> MDVVSLDKPFMYFEEIDNELDYEPESANEVAKKLPYQGQLKLLLGELFFLSKLQRHGILDGATVVYIGSAPGTHIRYLRDHFYNLGVIIKWMLIDGRHHDPILNGLRDVTLVTRFVDEEYLRSIKKQLHPSKIILISDVASAAGGNEPSTADLLSNYALQNVMISILNPVASSLKWRCPFPDQWIKDFYIPHGNKMLQPFAPSYSAEMRLLSIYTGENMRLTRVTKSDAVNYEKKMYYLNKIVRNKVVVNFDYPNQE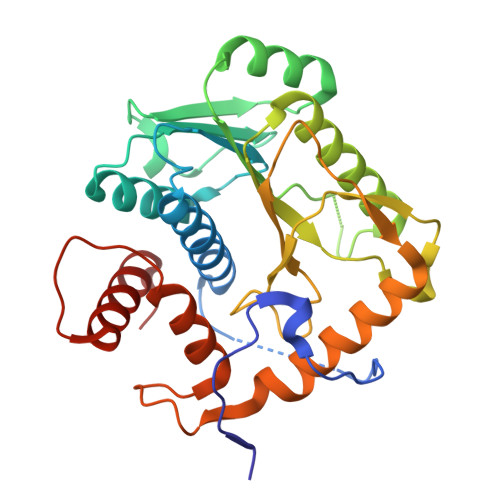YDYFHMYFMLRTVYCNKTFPTTKAKVLFLQQSIFRFLNIP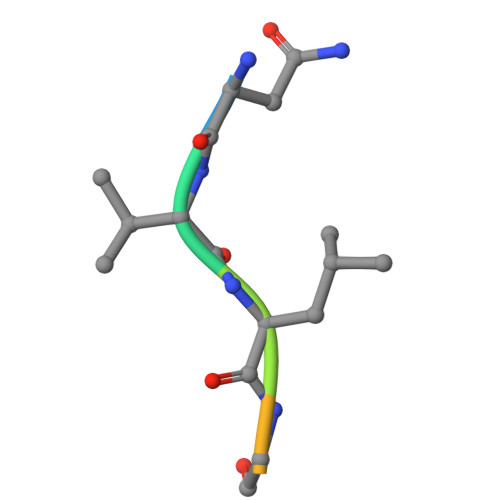> NVLGFTQ>ATTHLDVCAVVPAAGFGRRMQTECPKQYLSIGNQTILEHSVHALLAHPRVKRVVIAISPGDSRFAQLPLANHPQITVVDGGDERADSVLAGLKAAGDAQWVLVHDAARPCLHQDDLARLLALSETSRTGGILAAPVRD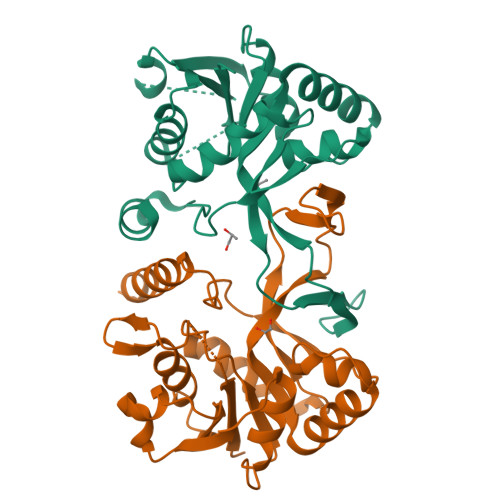TMKRAEPGKNAIAHTVDRNGLWHALTPQFFPRELLHDCLTRALNEGATITDEASALEYCGFHPQLVEGRADNIKVTRPEDLALAEFYLTRTIHQENT[2x]> FNCTSSSATVHWLGDKPTYHAGVTFGLPWPQGKYRPQETSFSLTGDTEDKSELQSWATGYWADGSLKWTAHAIAESNQIYDQYTVTASSLGCVKSSSSSSESSAPNSSIVVTDNSDALTVNTGEVAVSFPKGGNVIIGDIKTKSGKVIGANGRLVLQSQDSVPDNFDNRANSPIQYSNFDGNINEVFVNQTSARTLVTVRGNHTVTDGTDHDPWLPFVVRFYLYANSATIKVMHSIVFDGDENDFITGLGIRFDVPLKGEEYYDRHIRFAGVDGGIFNEAVQGITGLRRDPGEEIRAAQFAGQKLADTETWEPRVSTRLKWIPTWADYGLTQLTADGFGLKKRTKAGQSWVNIPSGTRAEGLAYLGGATQGGLAVGLRDFWKRYPVGLDISNAASDTGELTLWLYSPAAEPLDLRPFHDGLGQDGYEDQLDALEITYEDWEPGFDTPYGIARTSEVYLFAFDQTPTSDKLASLTAYMNDPPVLVAEPKYIHETQALGEYWA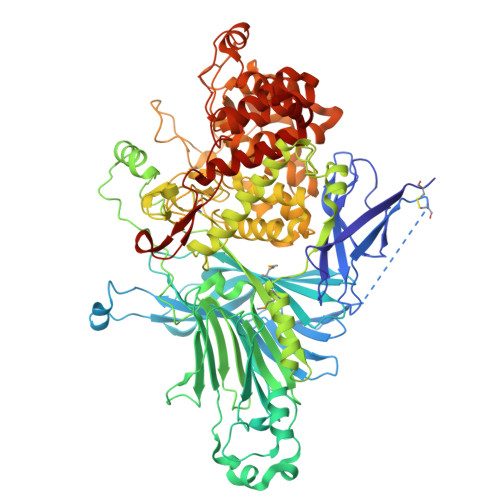LPGSASPAAATLEDRLQFIFDFYKGQIEQRRWYGFLDYGDFMHTYDPDRHTWRYDVGGYAWDNSELSPDLFFWLYFLRTGSKDAYRFAEALTRHTGEVDVYHIGDWKGLGTRHGVQHWSDSAKQARISQPQYRKYFFYLSGGDERVGELLEELLDTDKTYGELDPQRKVRTDGWEPSPNSTVSFGLGTDWSGLAAGWLIEWERRGPRWEEAKTKLTNTIAGIANLTNGFVTGSGLYDPVTWTLGPPPSDPGNRGNVSISHLNAVFGLPEVVSEAIAYLADDIPKGFKQAWLDYCYYYHASASEQKDRYGVSFSKISLLQAHSRLAAYAAYETKNKTLALRAWKDFYASDGLLPDAPWNITHVDGSDVLVPVDEAAWLATNDIAQYGLAVIQNLAYVSDSLDDYQS> MRGSHHHHHHGSTANPSLVLNKIDDISFETYDAPEISEPTDVLVQVKKTGICGSDIHFYAHGRIGNFVLTKPMVLGHESAGTVVQVGKGVTSLKVGDNVAIEPGIPCRFCDECKSGHYNLCPHMAFAATPNSKEGEPNPPGTLCKYFKSPEDFLVKLPDHVSLELGALVEPLSVGVHASKLGSVAFGDYVAVFGAGPVGLLAAAVAKTFGAKGVIVVDIFDNKLKMAKDIGAATHTFNSKTGGSEELIKAFGGNVPNVVLECTGAEPCIKLGVDAIAPGGRFVQVGNAAGPVSFPITVFAMKELTLFGSFRYGFNDYKTAVGIFDTNYQNGRENAPIDFEQLITHRYKFKDAIEAYDLVRAGKGAVKCLIDGPE

Xylitol dehydrogenase (XDH) catalyzes the NAD+-dependent oxidization of xylitol into d-xylulose, and belongs to a zinc-dependent medium-chain dehydrogenase/reductase family. This protein family consists of enzymes with one or two zinc atoms per subunit, among which catalytic zinc is necessary for the activity. Among many XDHs from yeast and fungi, XDH from Pichia stipitis is one of the key enzymes for bioethanol production by lignocellulosic biomass, and possesses only a catalytic zinc atom. Xylitol is then oxidized by xylitol dehydrogenase (XDH; EC 1.1.1.9) to give d-xylulose.

The so-called PsXDHC4 mutant was previously constructed by substituting Ser96, Ser99, and Tyr102 with cysteine residues in the wild-type (WT) enzyme. On the other hand, the introduction of four cysteine residues provided additional zinc-binding sites and significantly increased thermostability. Each monomer contained a bidomain architecture composed of a large “catalytic domain” (Thr2-Val163 and Arg300-Pro362) and a smaller “coenzyme-binding domain” (Gly164-Phe299), with a large cleft separating them. The former consisted of an α/β fold with a similar structure to that in other MDR enzymes, and the latter had the characteristic α/β Rossmann fold. Analytical size-exclusion chromatographic studies demonstrated that PsXDHC4 formed a homotetramer in solution. The four subunits (A–D) in the biological tetramer generated from crystallographic 222 symmetry were regarded as a dimer of identical A/B and C/D dimers. An anomalous difference Fourier map using data collected at the K-edge of zinc (wavelength of 1.280 Å) showed two clear peaks within the electron density map of PsXDHC4. Catalytic zinc was coordinated by interactions with Cys41 (distance of 2.3 Å), His66 (2.3 Å), Glu67 (2.2 Å), and a water molecule (Wat6; 2.6 Å). The second zinc atom was bound within a loop that protruded from the catalytic domain of PsXDHC4, at which it was ligated by the enzyme residues Cys96, Cys99, Cys102, and Cys110 (distance of 2.3 Å). Superimposition to the crystal structures of other MDR enzymes revealed that this zinc atom was equivalent to (inherently bound) structural zinc, and there was no significant difference in their binding loops regardless of zinc.>UGGUGU[8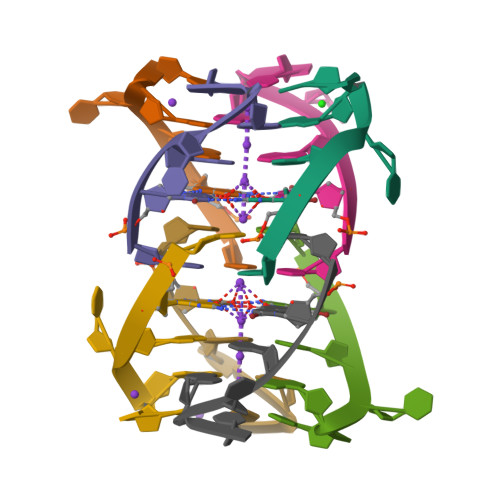x]4-{6-[(2S)-4-(2,4-diamino-6-ethylpyrimidin-5-yl)but-3-yn-2-yl]-2H-1,3-benzodioxol-4-yl}benzoic acid | C24 H22 N4 O4 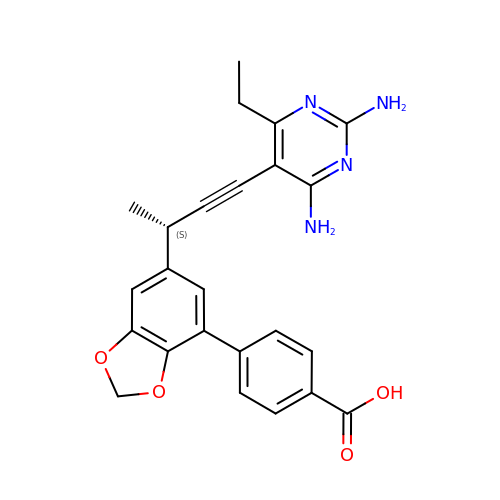| NQHZOWBSMCFILX-CYBMUJFWSA-N> GPGSD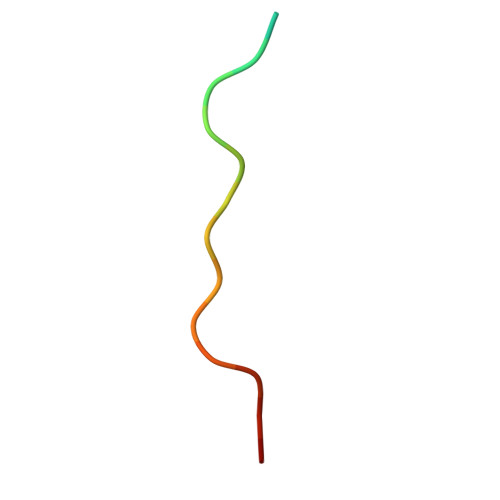RPPPYVAPPSYEG>MAMHPRKDWYELTRATNWTPSYVTEEQLFPERMSGHMGIPLEKWESYDEPYKTSYPEYVSIQREKDAGAYSVKAALERAKIYENSDPGWISTLKSHYGAIAVGEYAAVTGEGRMARFSKAPGNRNMATFGMMDELRHGQLQLFFPHEYCKKDRQFDWAWRAYHSNEWAAIAAKHFFDDIITGRDAISVAIMLTFSFETGFTNMQFLGLAADAAEAGDYTFANLISSIATDESRHAQQGGPALQLLIENGKREEAQKKVDMAIWRAWRLFAVLTGPVMDYYTPLEDRSQSFKEFMYEWIIGQFERSLIDLGLDKPWYWDLFLKDIDELHHSYHMGVWYWRTTAWWNPAAGVTPEERDWLEEKYPGWNKRWGRCWDVITENVLDDRMDLVSPETLPSVCNMSQIPLVGVPGDDWNIEVFSLEHNGRLYHFGSEVDRWVFQQDPVQYQNHMNIVDRFLAGQIQPMTLDGALKYMGFQSIEEMGKDAHDFAWADKCKPAMKKSA[2x];>[2x]MSFESKKPMRTWSHLAEMRKKPSEYDIVSRKLHYSTNNPDSPWELSPDSPMNLWYKQYRNASPLKHDNWDAFTDPDQLVYRTYNLMQDGQESYVQSLFDQFNEREHDQMVREGWEHTMARCYSPLRYLFHCLQMSSAYVQQMAPASTISNCCILQTADSLRWLTHTAYRTHELSLTYPDAGLGEHERELWEK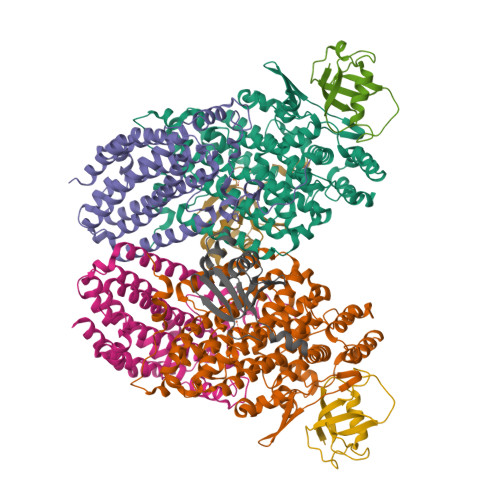EPGWQGLRELMEKQLTAFDWGEAFVSLNLVVKPMIVESIFKPLQQQAYENNDTLLPLLIDSQLKDAERHSRWSKALVKHALENPDNHAVIEGWIEKWRPLADRAAEAYLSMLSSDILHAQYLERSTSLRASILTV;>[2x]MSAFPVHAAFEKDFLVQLVVVDLNDSMDQVAEKVAYHCVNRRVAPREGVMRVRKHRSTELFPRDMTIAESGLNPTEVIDVVFEE;>[2x]MSTLAQQALHNNNVGPIIRAGDLVEPVIETAEIDNPGKEITVEDRRAYVRIAAEGELILTRKTLEEQLGRPFNMQELEINLASFAGQIQADEDQIRFYFDKTM>[6x]MRGSHHHHHHGSMDKNIIIGAMTALITPFKNGKVDEQSYARLIKRQIENGIDAVVPVGTTGESATLTHEEHRTCIEIAVETCKGTKVKVLAGAGSNATH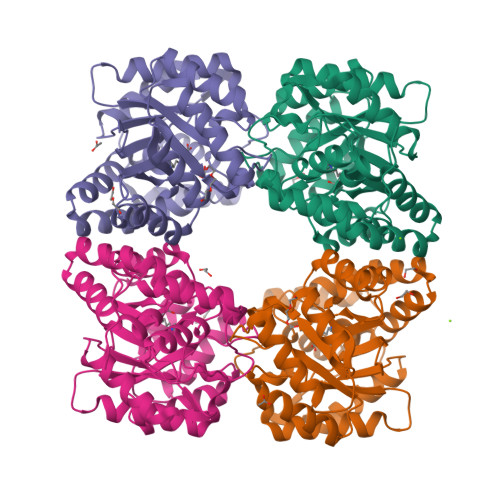EAVGLAKFAKEHGADGILSVAPFYNKPTQQGLYEHYKAIAQSVDIPVLLYNVPGRTGCEISTDTIIKLFRDCENIYGVKEASGNIDKCVDLLAHEPRMMLISGEDAINYPILSNGGKGVISVTSNLLPDMISALTHFALDENYKEAKKINDELYNINKILFCESNPIPIKTAMYLAGLIESLEFRLPLCSPSKENFAKIEEVMKKYKIKGF>PMFIVNTNVPRASVPDGFLSELTQQLAQATGKPPQYIAVHVVPDQLMAFGGSSEPCALCSLHSIGKIGGAQNRSYSKLLCGLLAERLRISPDRVYIAYYDMNAANVGW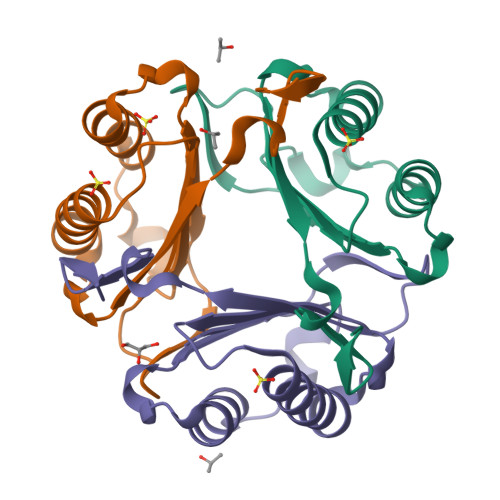NNSTFA[3x]>[3x]QPRRPGQTAREEILDAA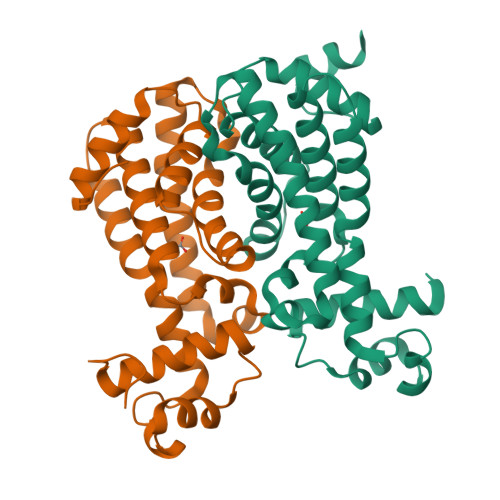AELFTTHGYGSTSTRRIADEVGVRQASLYHHFATKDDILDALLAGTVDEPLELAHGLLGESGPAAPRLHALVIYDASQLCAGRWNLGALYLLPELRTDRFAPFRRRRAELRSAYRSLAAAVIAECGGPPEADDLPFRLVESVINSRSDDAVVPPEQPWVIGEGALRVLGFDGDFAELAAATASRLGVRPPGRAARHHHHH> GPHMSAPNPKAFPLADAALTQQILDVVQQAANLRQLKKGANEATKTLNRGISEFIIMAADCEPIEILLHLPLLCEDKNVPYVFVPSRVALGRAC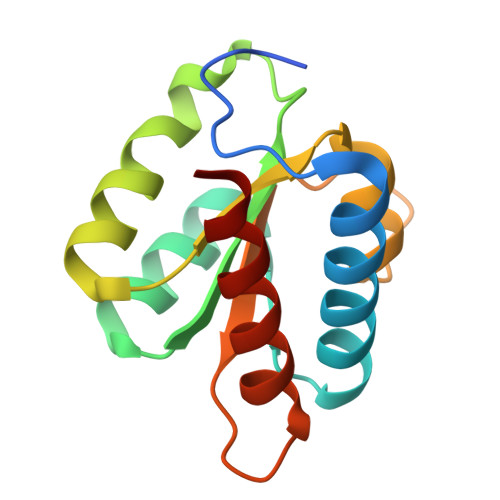GVSRPVIAASITTNDASAIKTQIYAVKDKIETLLI bromopromazine | C17 H19 Br N2 S | 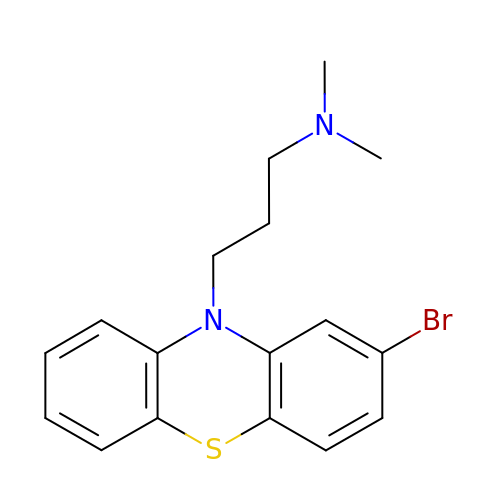MEYGNYCKJKFOTR-UHFFFAOYSA-N> PLGSVRWARALYD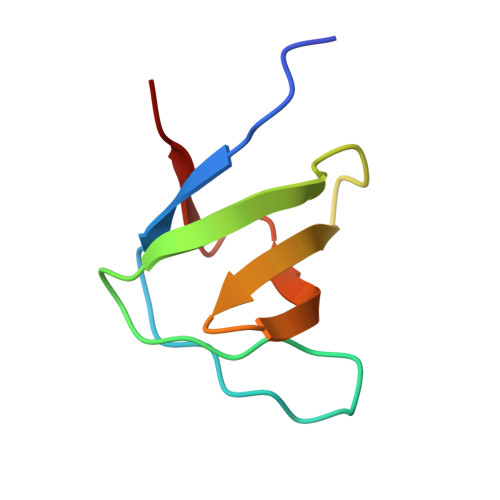FEALEEDELGFRSGEVVEVLDSSNPSWWTGRLHNKLGLFPANYVAPMMR>[4x]VKSKAKKTVDKHSDEYKIRRERNNIAVRKSRDKAKMRNLETQH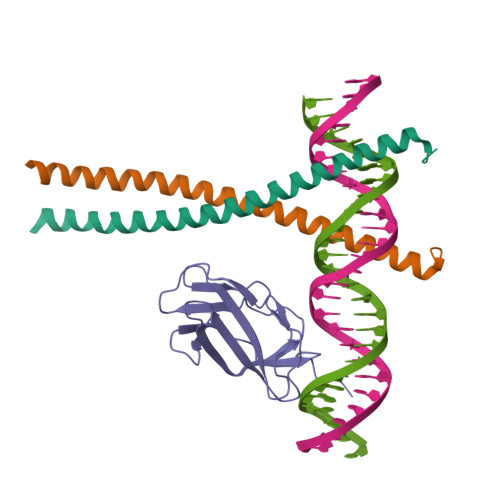KVLELTAENERLQKKVEQLSRELSTLRNLFKQLPEPLLASSGHC;>[2x]GELVRTDSPNFLCSVLPTHWRCNKTLPIAFKVVALGDVPDGTLVTVMAGNDENYSAELRNATAAMKNQVARFNDLRFVGRSGRGKSFTLTITVFTNPPQVATYHRAIKITVDGPREPRRHRQK> GSHMAVQIGFLLFPEVQQLELTGPHDVLASLPDVQVHLIWKEPGPVVASSGLVLQATTSFADCPPLDVICIPGGTGVGALMEDPQALAFIRQQAARARYVT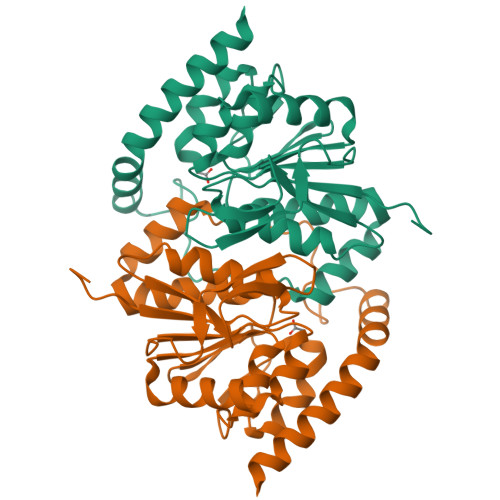SVCTGSLVLGAAGLLQGKRATTHWAYHELLAPLGAIPVHERVVRDGNLLTGGGITAGIDFALTLAAELFDAATAQRVQLQLEYAPAPPFNAGSPDTAPASVVQQARQRAADSLHKRREITLRAAARLAAG> MSWATRLLRMSSPRLGLLPLGRSVKLGGAKERVSFSQFFDSEYFWTKANVGPFFLFLFTSPFWYQGIKTVYASCRYRKL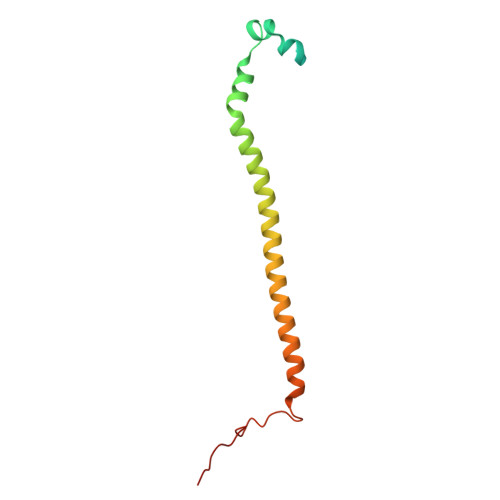NEREIISDRYTWLHERMLEDEVERVLLEQVPAGGFDKTRPGLLLGPSTL>GPGFDYAVAMAKRNIVTATTSKGEFTMLGVHDNVAILPTHASPGESIVIDGKEVEILDAKALEDQAGTNLEITIITLKRNEKFRDIRPHIPTQITE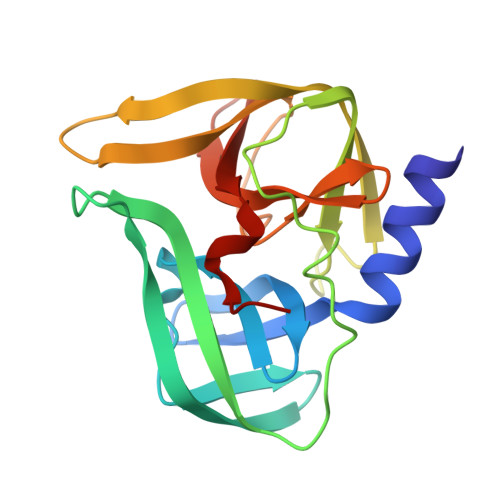TNDGVLIVNTSKYPNMYVPVGAVTEQGYLNLGGRQTARTLMYNFPTRAGQCGGVITCTGKVIGMHVGGNGSHGFAAALKRSYFTQSQ[2x]> AKPLSGFSQIRHEIPMLSLDNAFSDAEFNAFVKRIEDRLILLPKPLTFCCEPKLDGLAVSILYVNGELTQAATRGDGTTGEDITANIRTIRNVPLQLLTDNPPARLEVRGEVFMPHAGFERLNKYALEHNEKTFANPRNAAAGSLRQLDPNITSKRPLVLNAYGIGIAEGVGLPTTHYARLQWLKSIGIPVNPEIRLCNGADEVLDFYQDIQNKRSSLGYDIDGTVLKINDIALQNEL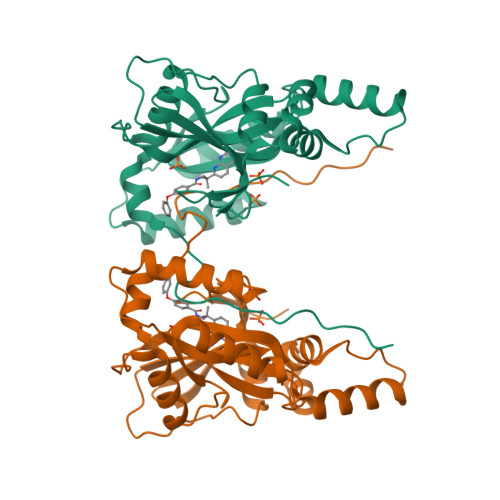GFISKAPRWAIAYKFPAQEELTLLNDHHHHHH(2S,5',S)-2-AMINO-3-(3-CARBOXY-2-ISOXAZOLIN-5-YL)PROPANOIC ACID | C7 H10 N2 O5 | 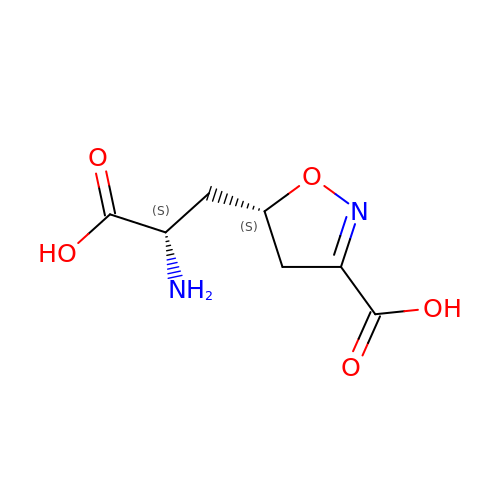AUXNPKGXCSBLJK-IMJSIDKUSA-N> SNAMQVITSVKEAKQIVKDWKSHQLSIGYVPTMGFLHDGHLSLVKHAKTQDKVIVSIFVNPMQFGPNEDFSSYPRDLERDIKMCQDNGVDMVFIPDATQMYLKNFSTYVDMNTITDKLCGAKRPGHFRGVCTVLTKFFNILNPDIVYMGQKDAQQ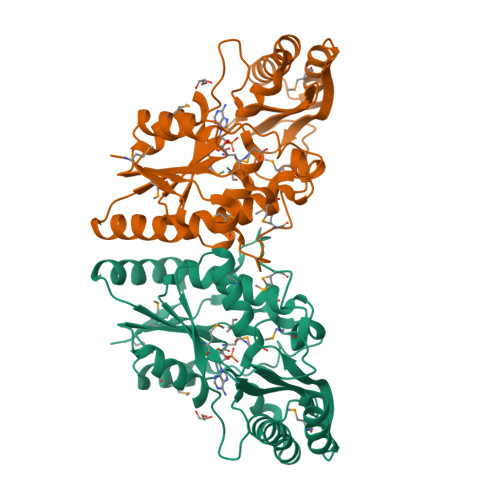CVVVRHMVDDLNFDLKIQICPIIREEDGLAKSSRNVYLSKEERKASLAISQSIFLAEKLVREGEKNTSKIIQAMKDILEKEKLIKIDYIELVDFNTMENIENITDNVLGAVAAFVGKTRLIDNFLVQGLK>[2x]ERMILIRG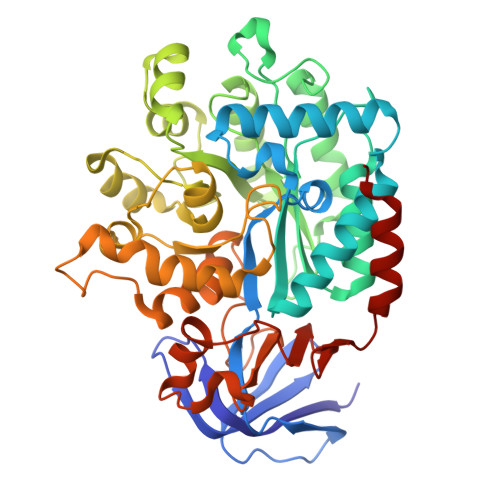LTRVITFDDQERELEDADILIDGPKIVAVGKNLSDRSVSRTIDGRGMIALPGLINSHQHLYEGAMRAIPQLERVTMASWLEGVLTRSAGWWRDGKFGPDVIREVARAVLLESLLGGITTVADQHPFFPGATADSYIDATIEAATDLGIRFHAVRSSMTLGKSEGGFCDDLFVEPVDRVVQHCLGLIDQYHEPEPFGMVRIALGPCGVTHDKPELFEAFAQMAADYDVRLHTHFYEPLDAGMSDHLYGMTPWRFLEKHGWASDRVWLAHAVVPPREEIPEFADAGVAIAHLIAPDLRLGWGLAPIREYLDAGITVGFGTTGSASNDGGNLLGDLRLAALAHRPADPNEPEKWLSARELLRMATRGSAECLGRPDLGVLEEGRAADIACWRLDGVDRVGVHDPAIGLIMTGLSDRASLVVVNGQVLVENERPVLADLERIVANTTALIPKNL>MTERKPEVIITYCTQCQWLLRAAWLAQELLSTFSDDLGKVSLEPATGGAFRITCDGVQIWERKADGGFPEAKVLKQRVRDQIDPERDLGHNDRT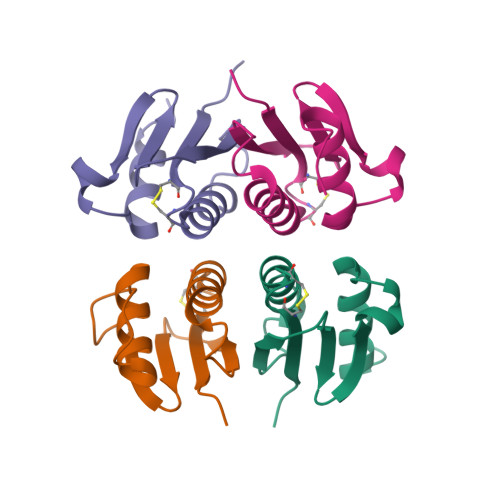QLEHHHHHH[8x]>AIEFDIQESKILKGVYIITPNKFRDLRGEIWTAFTDEYLSKLVPDGIKFKHDKFINSHFNVLRGIHGDVKTYKLVTCVYGEVHQVVVDCRKDSPTYLKWEKFIISYKNQQLILLPPNMGNSHYVS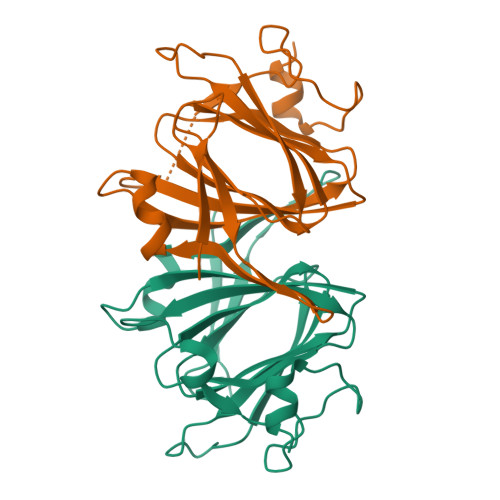SKEAVYYYKLAYEGEYMDAPDQFTYAWNDERIGIDWPTNTPILSDRDILATK[4x]>MHHHHHHSSGMNWTVDIPIDQLPSLPPLPTDLRTRLDAALAKPAAQQPTWPADQALAMRTVLESVPPVTVPSEIVRLQEQLAQVAKGEAFLLQGGDCAETFMDNTEPHIRGNVRALLQMAVVLTYGASMPVVKVARIAGQYAKPRSADIDALGLRSYRGDMINGFAPDAAAREHDPSRLVRAYANASAAMNLVRALTSSGLASLHLVHDWNREFVRTSPAGARYEALATEIDRGLRFMSACGVADRNLQTAEIYASHEALVLDYERAMLRLSDGDDG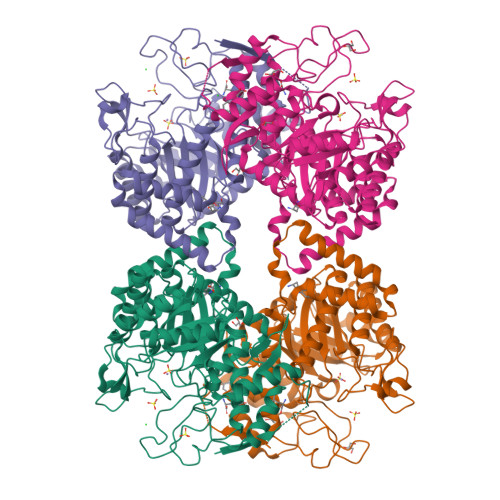EPQLFDLSAHTVWIGERTRQIDGAHIAFAQVIANPVGVKLGPNMTPELAVEYVERLDPHNKPGRLTLVSRMGNHKVRDLLPPIVEKVQATGHQVIWQCDPMHGNTHESSTGFKTRHFDRIVDEVQGFFEVHRALGTHPGGIHVEITGENVTECLGGAQDISETDLAGRYETACDPRLNTQQSLELAFLVAEMLRD[2x]N-ACETYL-L-CYSTEINE | 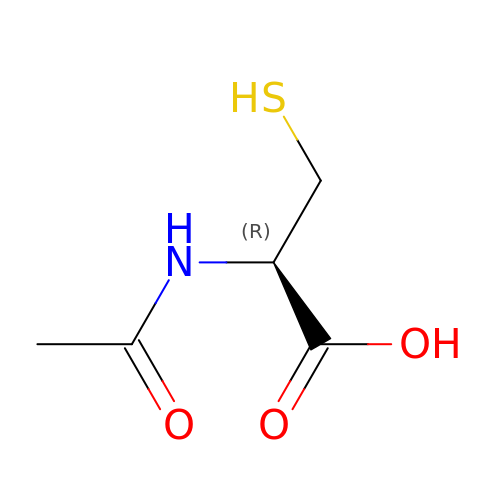C5 H9 N O3 S | PWKSKIMOESPYIA-BYPYZUCNSA-N Phage satellite P4 polarity suppression protein, Psu, a building block of the viral capsid, inhibits hexameric transcription termination factor, ρ, by presently unknown mechanisms. The ρ hexamer adopts an NTPase-inactive, washer-like, open-ring conformation until NTPs (preferentially ATP) are engaged and RNA is bound at the SBS, leading to ring closure and RNA entrapment inside the ring. Our cryogenic electron microscopy structures of ρ-Psu complexes show that Psu dimers clamp two inactive, open ρ rings and promote their expansion to higher-oligomeric states. ATPase, nucleotide binding and nucleic acid binding studies revealed that Psu hinders ρ ring closure and traps nucleotides in their binding pockets on ρ.

A ρ variant harboring a P167L substitution has been observed to bind Psu more tightly than wt ρ38,43. Incorporation of this additional ρP167L subunit leads to an interlocking of the two ρP167L rings, due to refolding and domain swapping of the central ρP167L subunits, most likely explaining the increased ρP167L-Psu affinity (Supplementary Discussion). Such refolding and domain-swapping in ρP167L only occurs in complex with Psu, as it is not observed in a cryoEM structure of isolated ρP167L. The final percentage of hydrolyzed ATP (reaction amplitude) was comparable for ρwt and ρP167L, but the ATP turnover rate of ρP167L was approximately doubled compared to ρwt. In the absence of Psu, ρwt and ρP167L exhibited similar Kd’s for mant-ATPγS (9.3 µM and 14.0 µM, respectively). The slightly lower mant-ATPγS affinity of ρP167L is due to a two-fold higher dissociation rate, which likely arises because the residue substitution renders the nucleotide-binding site more dynamic, as indicated by the lower thermal stability of ρP167L. The increased nucleotide dissociation constant may enable faster ATP turnover, consistent with the observed elevated ATPase rate of ρP167L compared to ρwt. While ρP167L does not exhibit defects in laboratory assays, the proline at the 167-equivalent position is invariant, perhaps to provide higher ρ stability.

>[6x]MNLTELKNTPVSELITLGENMGLENLARMRKQDIIFAILKQHAKSGEDIFGDGVLEILQDGFGFLRSADSSYLAGPDDIYVSPSQIRRFNLRTGDTISGKIRPPKEGERYFALLKVNEVNFDKPENARNKILFENLTPLHANSRLRMERGNGSTEDLTARVLDLASLIGRGQRGLIVAPPKAGKTMLLQNIAQSIAYNHPDCVLMVLLIDERPEEVTEMQRLVKGEVVASTFDEPASRHVQVAEMVIEKAKRLVEHKKDVIILLDSITRLARAYNTVVPASGKVLTGGVDANALHRPKRFFGAARNVEEGGSLTIIATALIDTGSKMDEVIYEEFKGTGNMELHLSRKIAEKRVFPAIDYNRSGTRKEELLTTQEELQKMWILRKIIHPMGEIDAMEFLINKLAMTKTNDDFFEMMKRS>MAMDLFQDKVEAFTGPTMGSTYTVKYVRSGDGPAKEVLHGEVEAILGQLDKQLSTYRSDSDVERFNALPAGSCEPMPDMVRELVAAGSQLSADSDGAFDLTLEPLLNLWGFGPQGRGERVPSAEDISAARALTGQQHLSIDGDRLCKAVALQLDFNSIAAGYAVDLVIDRLKAL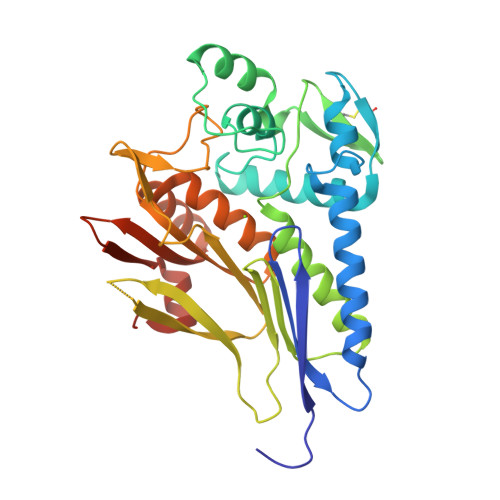GVQSYLVEITGELKAEGRKPDGSPWRIAIEAPRDDQRVAQKIVELDGMGVSTSGDYRNYFERDGRRYSHTLDPQSGQPIEHHLAAVTVIDKSTLRADGLSTALMVLGPEKGLALAERNGIAAFFVVREGQGFVTTSTKAFDELFGAGVEQVEHHHHHH[8x]> FDDVVVSRQEQSYVQRGMVNFLDEEMHKLVKRFRDMRWNLGPGFVFLLKKVNRERMMRYCMDYARYSKKILQLKHLPVNKKTLTKMGRFVGYRNYGVIRELYADVFRDVQGFRGPKMTAAMRKYSSKDPGTFPCK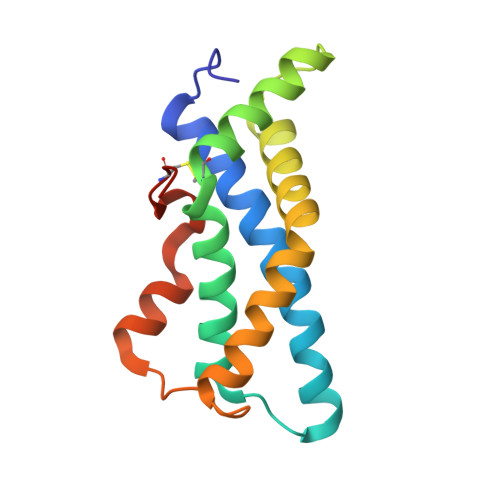NEKRRG>[2x]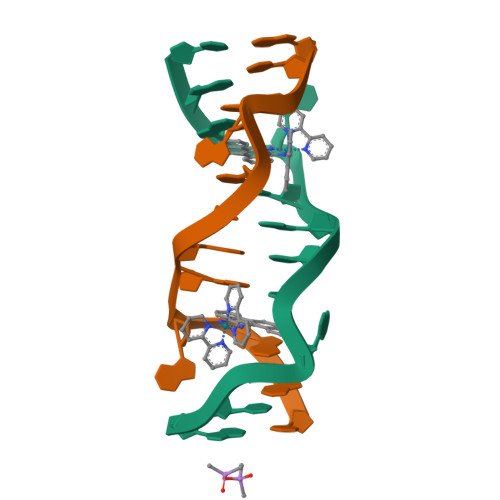CGGAAATTACCG> MSVNTSF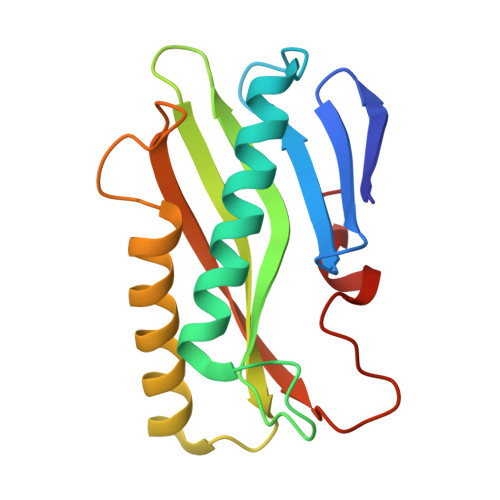LSPSLVTIRDFDKGQFAVLRIGRTGFPADKGDIDLCLSKMDGVLAAQLYLGNPREPGFKGPHIRIRCVDIDDKHTYNAMVYVDLIVGTGASEVERETAEERARRALAVALRVDEADEHSCVTQFEMKLREELLSSDSFHPDKDEYYKDFL>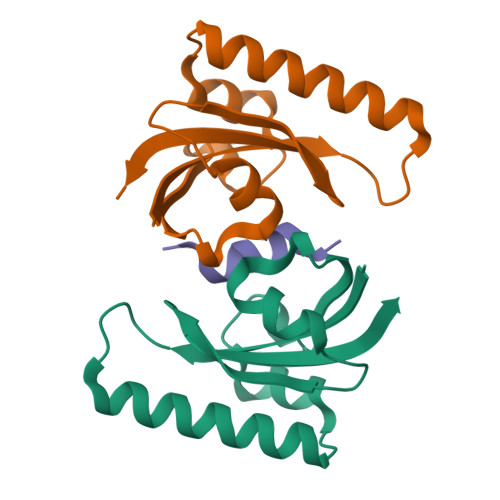[4x]TELNLSHILIPLPENPTSDQVNEAESQARAIVDQARNGADFGKLAIAHSADQQALNGGQMGWGRIQELPGIFAQALSTAKKGDIVGPIRSGVGFHILKVNDLR;>[2x]NFTLKFWDIFRK>[3x]MRIVAADTGGAVLDESFQPVGLIATVAVLVEKPYKTSKRFLVKYADPYNYDLSGRQAIRDEIELAIELAREVSPDVIHLNSTLGGIEVRKLDESTIDALQISDRGKEIWKELSKDLQPLAKKFWEETGIEIIAIGKSSVPVRIAEIYAGIFSVKWALDNVKEKGGLLVGLPRYMEVEIKKDKIIGKSLDPREGGLYGEVKTEVPQGIKWELYPNPLVRRFMVFEITSKSHHHH

Here, we report the crystal structures of PhoExo I, which shares 76% amino acid sequence identity with PfuExo I. In this study, we determined three substrate-free structures of PhoExo I and four structures of PhoExo I in complexes with ssDNAs. PhoExo I forms a trimer in solution similar to PfuExo I. The 3′-5′ exonuclease assay of PhoExo I showed that PhoExo I cleaved an ssDNA from its 3′-end at every two nucleotides, and the cleavage stopped at the third to fifth nucleotide from the 5′-end. PhoExo I is predicted to utilize a DEDE (RNase HIII)-type catalytic motif for the hydrolysis of ssDNA. PhoExo I is a novel RNase H superfamily protein.

To examine the mechanisms of ssDNA recognition and cleavage by PhoExo I, we cocrystallized PhoExo I with poly-dA, poly-dC and poly-dT. To prevent the degradation of ssDNA during the cocrystallization, we used the D80N mutant of PhoExo I; the corresponding mutation was previously utilized in a cocrystallization study of the B. halodurans RNase HI―DNA/RNA hybrid complex. In this study, we determined the crystal structures of PhoExo I in complexes with poly-dA, poly-dC and poly-dT at 2.05 Å, 2.50 Å and 2.05 Å, respectively. Each crystal contained one PhoExo I trimer and three oligonucleotides in the asymmetric unit. Although the overall structures of the PhoExo I―ssDNA complexes were nearly identical, PhoExo I formed some base-specific interactions with ssDNAs. In addition, the base groups of the poly-dC and poly-dT formed direct hydrogen bonds with Arg55 and Arg104, and they formed water-mediated hydrogen bonds with Phe17 and Asn214. These interactions may support the substrate recognition of PhoExo I; PhoExo I prefers poly-dT because PhoExo I forms the largest number of base-specific interactions with poly-dT compared to poly-dA and poly-dC. Although Lys136 formed no direct hydrogen bonds with the phosphate groups of the ssDNAs, except in the PhoExo I―poly-dC complex, the 3′-5′ exonuclease activity of PhoExo I was significantly decreased by the K136A mutation. The structures of the PhoExo I―ssDNA complexes showed that the deoxyribose groups of the substrate DNA contact the hydrophobic region of the active site pocket. The PhoExo I―ssDNA structures determined in this study are predicted to present the distributive cleavage state of PhoExo I. In this state, PhoExo I recognizes ssDNA only at the active site pocket that accommodates the 3′-OH terminal 4 nt of ssDNA, so the 5′-terminal 3 nt are disordered in the complex structures.> MAHMNTYLKPFELTLRCLGPVFIGSGEKRTSKEYHVEGDRVYFPDMELLYADIPAHKRKSFEAFVMNTDGAQATAPLKEWVEPNAVKLDPAKHRGYEVKIGSIEPRRASRGRGGRMTRKKLTLNEIHAFIKDPLGRPYVPGSTVKGMLRSIYLQSLVHKRT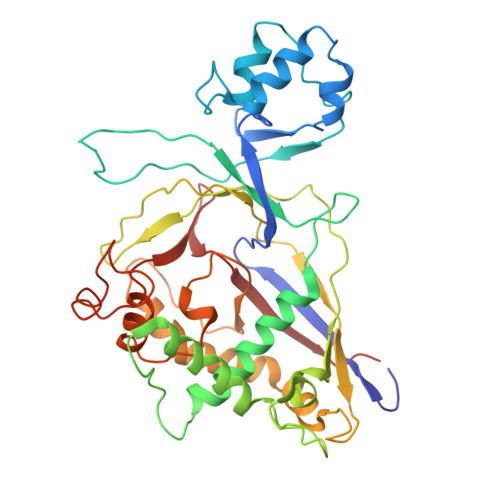AQPVRVPGHQTREHRQYGERFERKELRKSGRPNTRPQDAVNDLFQAIRVTDSPALRTSDLLICQKMDMNVHGKPDGLPLFRECLAPGTSISHRVVVDTSPTARGGWREGERFLETLAETAASVNQARYAEYRAMYPGVNAIVGPIVYLGGGAGYRSKTFVTDQDDMAKVLDAQFGKVVKHVDKTRELRVSPLVLKRTKIDNICYEMGQCELSIRRAE3-(1,3-benzothiazol-2-ylamino)-4-(2-methoxyphenyl)pyrrole-2,5-dione 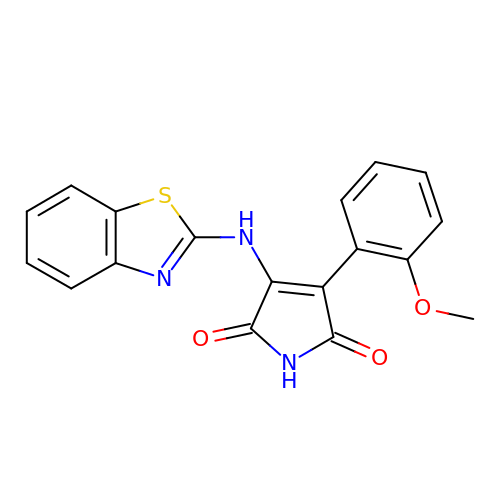| C18 H13 N3 O3 S | DKODQPUAYQCESR-UHFFFAOYSA-N> GFPCGESCVYLPCFTAAIGCSCKSKVCYKN;> GFPCGESCVYIPCFTAAIGCS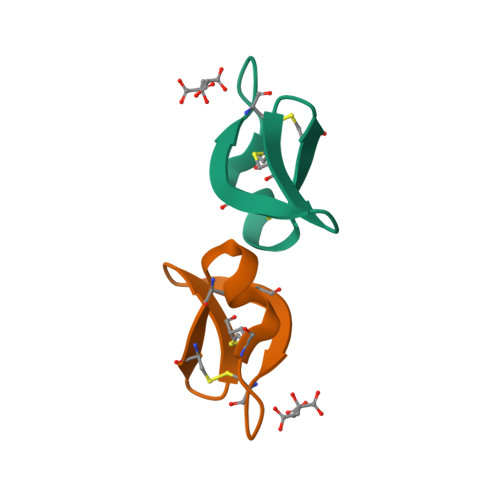CKSKVCYKN Staphylococcal picoviruses are a group of strictly lytic, short-tailed bacteriophages with compact genomes that are attractive candidates for therapeutic use. Here, we report the structure of the complete virion of S. epidermidis–infecting phage Andhra, determined using high-resolution cryo–electron microscopy, allowing atomic modeling of 11 capsid and tail proteins. The overall structure of the Andhra virion follows that of other phages in this group, with an isometric head (capsid) around 500 Å in diameter (vertex to vertex), connected to a 400-Å-long, straight tail surrounded by 12 appendages. The head has icosahedral symmetry, with the tail attached to a portal structure located at 1 of the 12 fivefold vertices.

(C) One asymmetric unit of the C6 tail reconstruction, comprising 12 copies of core protein (gp20), two copies of PP (gp17), two copies of tail stem protein (gp16), six copies (two trimers) of RBP (gp15), and two copies of the anchor protein (gp6). The Andhra portal consists of 12 copies of PP (gp17), arranged in a 150-Å-wide ring with C12 symmetry, with a 30-Å-wide central hole. The PP monomer consists of three domains: the wing (51 to 160 and 258 to 334), the stem (6 to 50, 161 to 186, and 234 to 257), and the clip (residues 187 to 233). The wing domain resides inside the capsid where it interacts with the portal-proximal core protein (gp20) and the DNA, while the clip domain connects with the tail stem protein (gp16). On the distal side of the portal, the dodecameric tail stem or collar protein, gp16, forms an elongated tube that comprises the main stem of the tail. A 128-residue insertion between amino acids 122 and 250 forms a twisted β-hairpin, creating a 150-Å-long tubular β barrel with an inner diameter of ≈32 Å that acts as a conduit for the DNA. The 12 appendages surrounding the tail correspond to trimers of RBP, the 609-residue product of ORF15 (gp15). The Andhra RBP consists of an N-terminal 36- to 38-residue loop followed by a 34- to 38-residue α-helical coiled-coil stem domain, connected to a 534-residue C-terminal β helix domain. The true start for gp6 is thus most likely at nucleotide 1887 (TTG). gp6 forms six asymmetric dimers that bridge the RBP trimers and the tail stem protein (gp16). Because the gp6 dimers appear to anchor the RBP trimers in place, we refer to this protein as the “RBP anchor” protein.

>[6x]MYINNGRINYNNEYGYRRGIYREPFYSDNADYNTNSKSYYDYLARFNGFIFELCDFVNGLADDIQKMKDTYEALTLSNTDVTYTVGQKGDFDTLNHCFEHIEDLIVQPKSIRVILLKDYMMREQLFLRDKRYNHITITSENDIVEAYETELNRQVEIKTNPIFRVKPLFYGINSTFPKIDFKLQNKDFSDTINCGFLMDNTTFEMTERGGSTHFNFIGLCGVNGSHIQTNYCDFSYNGNREQLEEYNKDQNMYGDGLRIFNSSLTGNYMTVNRCGEIGIHFSHGASGYIDFTEARFNGHHGLMVTTGSQASARNCKITDTIDDNVVSYASSDIDLRSSDCSNSQTTYGVIATRSSNINFDKGIANGCGASGIMANRGCSIDATGATASRNKWHGVIASNNSKVDFTSGNANENGLDGIQCTHGSTVQARLSTTNGNKRNGVLAYAGDVYCQEINCDGNGRRGLEATRGGYVAAYGAKVSRSKDDNVLAYGSMISINEALIERAGRNGIEATRGGQIFADRITITGSGDFGILAYASKVFAEASNISGTKNEPVYATRGGEVTCFGSNISSNKTVYNVYNGSRIFTDKDHGYSTNVDPQTLSSKGLIILG;>[2x]MSYLDNDYIGKNKDVGLKVELTEDIDRRIMEHRNRFRRLIFNRYVEFLPLLINYTNQNSVGIDFLQLEIALRQGYQVVVGKARNGVIMILGYIQSMYYKNSNDFINNFNLTFNKRLTQDDITFIIPDYLRPDYALEIEYYDNCQSGDFIVLRNKPVNLNNDYQIIEHYCDELAEIILSRFSLIMQSKFSKIFLSDIQDETINQFINKLYNGAPFIKTDKYIDPEEDIIDLGSDFVTTALVEMKREYQNKVSELSNFLGVNSLAVDKESGVSDTEAKSNRSFTTSNSNIYLRGRNPFEMLNRRFNLDIHPYYDDEAISEMDIMNLKTDNFGGGKVE;>LSKHTTTLYEIIESELQRLGLNEFVNNDRIHFNDSKHAFMQKMLYFDDDVKQIVDHMFFKGFMFNDERIDRYFKESFTLRFLYREIGRQTVESFASQVLYITMTHEDYIYRVYGSDMYKYIEQVTDTQSQDLGKAIENAIEQGQTKDRQQDKGHEEYKDYEDTITKSFDDNRTAESTLPQSKVNIDVDNTVLDYADTNTISRDKNTSETVSEKTGTKDNTFDSLRNGESDTKRNTQSQNEMNRTGLTKQYLIDNLQKLYSMRDTIFKTYDKECFLHIW[2x];>LIIKHQMKLHLNELVDWAWRNGVTSEKFHSNNGSYVIFDHSAVVETYIINKNDLFNVTEEIEITLDKPIDYFLEKDMYGNYREHFGIAINDLLFLNTTVNIWLVNDDNSHILIYKDGKLIDEYMYHQFEYEANQNKHIYPNNKASGTYPHKTEQDVTPPKKQPDTKPLPPEEHTPKVRTIKTLNGTVMKDYTPVSSIQYVKSVGIIGDSVGKGAHASYNFGDYINEKTGAKIQNLSVSSATMSEVKDNNILNQAKQLKDNELVIIQGTDDDWLFNSNAGVEVGNKITDTKTYIGAFYKVVETVKENNPKAKIVVITPTKQAKIDDTGKVIRRDTDKNKKGYTLKTYVDSQVKATKDLGLALYNAYDDSLINPYDEKFRQSSMKDGLHPTKWGHEMMYYRIAETYHKNFD[2x];>[12x]MAEEEKIIKEEPTNEETEQPEKIESAEDVVTEPEKEVTEEKSEAFVQLEQRISSLEQRLNNLESQPQPTQESSDPNFEDKTVPTEVDDNQETDGIESSEEIKQMLNL> MARVAVLISGTGSNLQALIDSTREPNSSAQIDIVISNKAAVAGLDKAERAGIPTRVINHKLYKNRVEFDSAIDLVLEEFSIDIVCLAGFMRILSGPFVQKWNGKMLNIHPSLLPSFKGSNAHEQALETGVTVTGCTVHFVAEDVDAGQIILQEAVPVKRGDTVATLSERVKLAE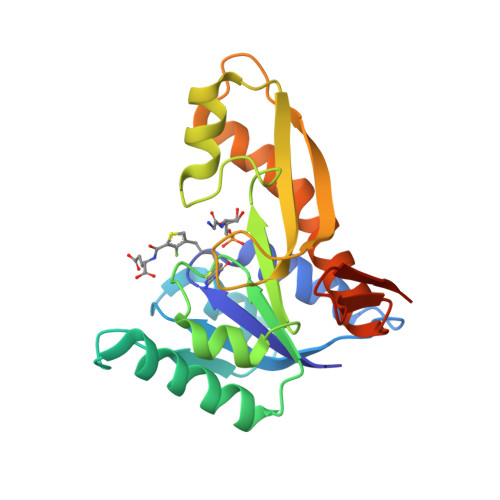HKIFPAALQLVASGTVQLGENGKICWVKEEHHHHHH>[4x]MSEQYSEINTDTLERVTEIFKALGDY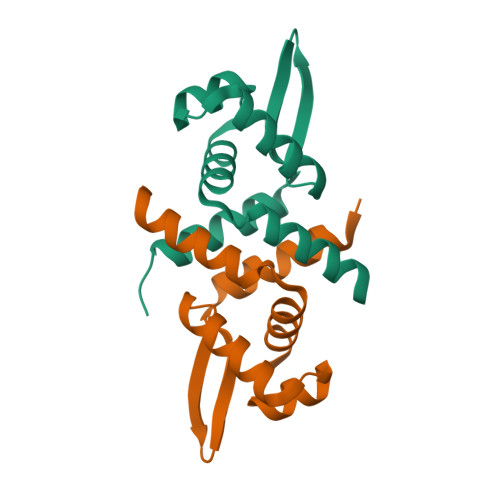NRIRIMELLSVSEASVGHISHQLNLSQSNVSHQLKLLKSVHLVKAKRQGQSMIYSLDDIHVATMLKQAIHHANHPKESGL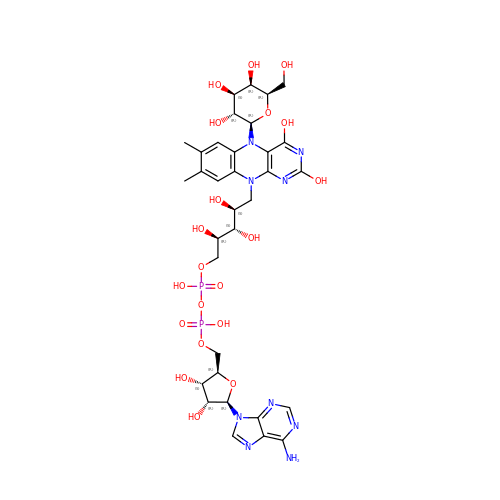[[(2~{R},3~{S},4~{R},5~{R})-5-(6-aminopurin-9-yl)-3,4-bis(oxidanyl)oxolan-2-yl]methoxy-oxidanyl-phosphoryl] [(2~{R},3~{S},4~{S})-5-[5-[(2~{R},3~{R},4~{S},5~{R},6~{R})-6-(hydroxymethyl)-3,4,5-tris(oxidanyl)oxan-2-yl]-7,8-dimethyl-2,4-bis(oxidanyl)benzo[g]pteridin-10-yl]-2,3,4-tris(oxidanyl)pentyl] hydrogen phosphate | C33 H45 N9 O20 P2 | KSCHBBHODWJJRH-MORZIXKLSA-N>MAMYQNMLVVIDPNQDDQPALRRAVYLHQRIGGKIKAFLPIYDFSYEMTTLLSPDERTAMRQGVISQRTAWIHEQAKYYLNAGVPIEIKVVWHNRPFEAIIQEVISGGHDLVLKMAHQHDRLEAVIFTPTDWHLLRKCPSPVWMVKDQPWPEGGKALVAVNLASEEPYHNALNEKLVKETIELAEQVNHTEVHLVGAYPVTPINIAIELPEFDPSVYNDAIRGQHLLAMKALRQKFGINENMTHVEKGLPEEVIPDLAEHLQAG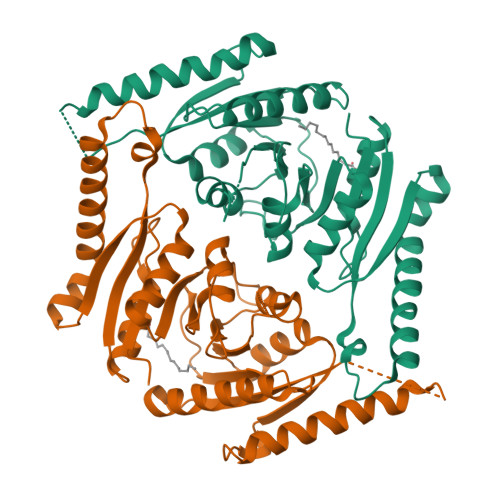IVVLGTVGRTGISAAFLGNTAEQVIDHLRCDLLVIKPDQYQTPVELDDEEDD[2x]Red algae utilise a megadalton-size light harvesting antenna called the red algal phycobilisome (PBS)—comprised of rod structures formed from stacked, hexameric protein-pigment rings emanating from a protein core that is poised above an integral membrane photosystem. Published cryo-EM maps for two red algal phycobilisomes contain clusters of unmodelled density homologous to the cryptophyte-αβ protomer. We modelled these densities, identifying a new family of scaffolding proteins related to red algal phycobilisome linker proteins that possess multiple copies of a cryptophyte-α-like domain. These domains bind to, and stabilise, a conserved hydrophobic surface on phycoerythrin β, which is the same binding site for its primary partner in the red algal phycobilisome, phycoerythrin α.

We call the family of scaffolding proteins CaRSPs (CALM repeat scaffolding proteins), where each CALM domain binds a PE β, stabilising and locating it within the red algal PBS. Further inspection of the deposited maps for the P. purpureum red algal PBS revealed evidence for continuous density linking clusters of cryptophyte-like PE β subunits together; three such clusters were identified, corresponding perfectly with the three candidate CaRSP sequences that we identified from P. purpureum. The other two clusters have three and two scaffolded PE β subunits which correspond to the predicted domain architecture of the sequences that we call CaRSP1 and CaRSP2, respectively. For the unmodelled region of LR6 and most of the remaining two CaRSPs, we built de novo models including models for the metamorphic N-terminal domain of the associated PE β subunits. Analysis of each CaRSP structure confirms that they are scaffolding proteins given that two have an anchoring domain and all CaRSPs make multiple contacts with red algal PBS rods as they weave between ‘lone’ PE β subunits.

> MWEQQRPRRCEAPAAPSSRPAERRAAARRSRAQLRMKQDDYEQWKTEFAGGFPGGEAFYKKWIEEGAKGDVPALEEELQPRSPNKKPTIYEEQMISNRGQQKGVDPTWKTLLAGGFPGGEFFFKKWIGEGAQGEVPNLDADLQPGSGSAKKTGKKEDADKSSPGGIMTPGRIMVPSGLGEEEETVDKEAPRPELYNKYFSADRLHKAPEILFEYNKTKYDRVGVRYTEVTSKASERFFPKSRMNRAPVIEISYREGAVSTASVSLSMPEISGPPALPFPVPKGDVTTTMVTDPTTGRLKLEFKVDGAAVSAYSDPRATEAYNKMIRK;>[2x]MLDAFSRVVVNSDAKAAYVGGSDLQALKSFIADGNKRLDAVNSIVSNASCMVSDAVSGMICENPGLISPGGNCYTNRRMAACLRDGEIILRYVSYALLAGDASVLEDRCLNGLKETYIALGVPTNSSIRAVSIMKAQAVAFITNTATERKMSFAAGDCTSLASEVASYFDRVGAAIS> SMDKLLLANWGLPKAVLEKYHSFGVKKMFEWQAECLLLGQVLEGKNLVYSAPTSAGKTLVAELLILKRVLEMRKKALFILPFVSVAKEKKYYLQSLFQEVGIKVDGYMGSTSPSRHFSSLDIAVCTIERANGLINRLIEENKMDLLGMVVVDELHMLGDSHRGYLLELLLTKICYITRKSASCQADLASSLSNAVQIVGMSATLPNLELVASWLNAELYHTDFRPVPLLESVKVGNSIYDSSMKLVREFEPMLQVKGDEDHVVSLCYETICDNHSVLLFCPSKKWCEKLADIIAREFYNLHHQAEGLVKPSECPPVILEQKELLEVMDQLRRLPSGLDSVLQKTVPWGVAFHHAGLTFEERDIIEGAFRQGLIRVLAATSTLSSGVNLPARRVIIRTPIFGGRPLDILTYKQMVGRAGRKGVDTVGESILICKNSEKSKGIALLQGSLKPVRSCLQRREGEEVTGSMIRAILEIIVGGVASTSQDMHTYAACTFLAASMKEGKQGIQRNQESVQLGAIEACVMWLLENEFIQSTEASDGTEGKVYHPTHLGSATLSSSLSPADTLDIFADLQRAMKGFVLENDLHILYLVTPMFEDW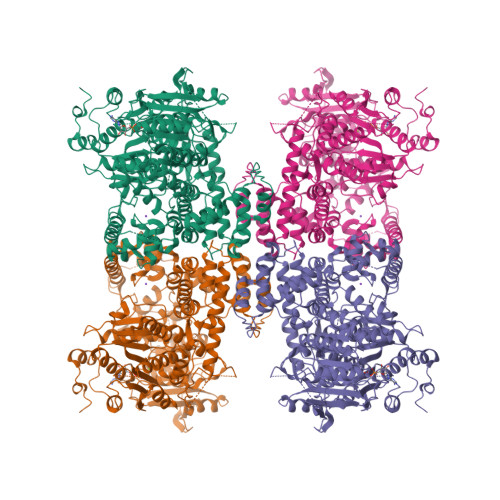TTIDWYRFFCLWEKLPTSMKRVAELVGVEEGFLARCVKGKVVARTERQHRQMAIHKRFFTSLVLLDLISEVPLREINQKYGCNRGQIQSLQQSAAVYAGMITVFSNRLGWHNMELLLSQFQKRLTFGIQRELCDLVRVSLLNAQRARVLYASGFHTVADLARANIVEVEVILKNAVPFKSARKAVDEEEEAVEERRNMRTIWVTGRKGLTEREAAALIVEEARMILQQDLVEM> MDDYKYQDNYGGYAPSDGYYRGNESNPEEDAQSDVTEGHDEEDEIYEGEYQGIPHPDDVKAKQAKMAPSRMDSLRGQTDLMAERLEDEEQLAHQYETIMDECGHGRFQWILFFVLGLALMADGVEVFVVSFALPSAEKDMCLSSSKKGMLGMIVYLGMMAGAFILGGLADKLGRKRVLSMSLAVNASFASLSSFVQGYGAFLFCRLISGIGIGGALPIVFAYFSEFLSREKRGEHLSWLGIFWMTGGLYASAMAWSIIPHYGWGFSMGTNYHFHSWRVFVIVCALPCTVSMVALKFMPESPRFLLEMGKHDEAWMILKQVHDTNMRAKGTPEKVFTVSNIKTPKQMDEFIEIQSSTGTWYQRWLVRFKTIFKQVWDNALYCVMGPYRMNTLILAVVWFAMAFSYYGLTVWFPDMIRYFQDEEYKSKMKVFFGEHVYGATINFTMENQIHQHGKLVNDKFTRMYFKHVLFEDTFFDECYFEDVTSTDTYFKNCTIESTIFYNTDLYEHKFINCRFINSTFLEQKEGCHMDLEQDNDFLIYLVSFLGSLSVLPGNIISALLMDRIGRLKMIGGSMLISAVCCFFLFFGNSESAMIGWQCLFCGTSIAAWNALDVITVELYPTNQRATAFGILNGLCKFGAILGNTIFASFVGITKVVPILLAAASLVGGGLIALRLPETREQVLM;> MRGSHHHHHHGSLVPRGSPFVNKQFNYKDPVNGVDIAYIKIPNAGQMQPVKAFKIHNKIWVIPERDTFTNPEEGDLNPPPEAKQVPVSYYDSTYLSTDNEKDNYLKGVTKLFERIYSTDLGRMLLTSIVRGIPFWGGSTIDTELKVIDTNCINVIQPDGSYRSEELNLVIIGPSADIIQFECKSFGHEVLNLTRNGYGSTQYIRFSPDFTFGFEESLEVDTNPLLGAGKFATDPAVTLAHQLIHAGHRLYGIAINPNRVFKVNTNAYYEMSGLEVSFEELRTFGGHDAKFIDSLQENEFRLYYYNKFKDIASTLNKAKSIVGTTASLQYMKNVFKEKYLLSEDTSGKFSVDKLKFDKLYKMLTEIYTEDNFVKFFKVLNAKTFLNFDKAVFKINIVPKVNYTIYDGFNLRNTNLAANFNGQNTEINNMNFTKLKNFTGLFEFYKLLCVRGIITSKTKSLDKGYNKALNDLCIKVNNWDLFFSPSEDNFTNDLNKGEEITSDTNIEAAEENISLDLIQQYYLTFNFDNEPENISIENLSSDIIGQLELMPNIERFPNGKKYELDKYTMFHYLRAQEFEHGKSRIALTNSVNEALLNPSRVYTFFSSDYVKKVNKATEAAMFLGWVEQLVYDFTDETSEVSTTDKIADITIIIPYIGPALNIGNMLYKDDFVGALIFSGAVILLEFIPEIAIPVLGTFALVSYIANKVLTVQTIDNALSKRNEKWDEVYKYIVTNWLAKVNTQIDLIRKKMKEALENQAEATKAIINYQYNQYTEEEKNNINFNIDDLSSKLNESINKAMININKFLNQCSVSYLMNSMIPYGVKRLEDFDASLKDALLKYIYDNRGTLIGQVDRLKDKVNNTLSTDIPFQLSKYVDNQRLLSTFTEYIKNIINTSILNLRYESNHLIDLSRYASKINIGSKVNFDPIDKNQIQLFNLESSKIEVILKNAIVYNSMYENFSTSFWIRIPKYFNSISLNNEYTIINCMENNSGWKVSLNYGEIIWTLQDTQEIKQRVVFKYSQMINISDYINRWIFVTITNNRLNNSKIYINGRLIDQKPISNLGNIHASNNIMFKLDGCRDTHRYIWIKYFNLFDKELNEKEIKDLYDNQSNSGILKDFWGDYLQYDKPYYMLNLYDPNKYVDVNNVGIRGYMYLKGPRGSVMTTNIYLNSSLYRGAKFIIKKYASGNKDNIVRNNDRVYINVVVKNKEYRLATNASQAGVEKILSALEIPDVGNLSQVVVMKSKNDQGITNKCKMNLQDNNGNDIGFIGFHQFNNIAKLVASNWYNRQIERSSRTLGCSWEFIPVDDGWGERPLVPPTPGSAWSHPQFEK

Botulinum neurotoxin A1 (BoNT/A1) belongs to the most potent toxins and is used as a major therapeutic agent. BoNTs and BoNT-like proteins share a common domain organization and are produced as precursors that are cleaved into a 50 kDa light chain (LC) and a 100 kDa heavy chain (HC) that with the exception of BoNT/Wo remain connected by a disulfide bond. The LC is a zinc metalloprotease that specifically cleaves soluble N-ethylmaleimide-sensitive-factor attachment receptor (SNARE) proteins. While the physiological functions of SV2 proteins remains to be determined, their best-established role is to act as receptors for several BoNTs (BoNT/A, /D, /E, and /F).

To elucidate how SV2B interacts with the toxin, we prepared SV2B complexes with the inactive full-length BoNT/A1 (in the presence of a 20 molar excess of ganglioside GT1b) and HCA1. Although applied in excess, GT1b was not detectable in the complex structure with the full-length toxin. The SV2B-BoNT/A1 and SV2B-HC structures revealed that the HC domain binds to the LD of SV2B, extending one β-sheet of the β-helix fold by the antiparallel β-hairpin located at the convex side between the two toxin HC subdomains. Unexpectedly, BoNT/A1 binding to SV2B resulted in a switch from the semi-closed to the open conformation, the domain arrangement that is observed in the crystal structure of the isolated, full-length toxin. Notably, based on our structure, in the open conformation, the HN and the LC are positioned far away from the plasma membrane or the synaptic vesicle membrane (~40 Å from the lipid bilayer margin), suggesting that this conformation prevents BoNT/A1 translocation. During intoxication, this state would correspond to that of a receptor-bound toxin on the cell-surface or after uptake into synaptic vesicle prior to acidification. Because in the open conformation of the SV2B-bound toxin the LC and HN are far away from the synaptic vesicle membrane, the role of this conformation appears to be the prevention of the interaction of the two domains with membranes and premature translocation before the toxin/receptor complex reaches its proper destination. Microscale thermophoresis (MST)-based experiments revealed a high-affinity interaction of SV2B with BoNT/A1 and HCA1, with very similar KD values of 110 nM and 180 nM, respectively.> MLFAPTIKAQADTVPLPAPIIEAFPVEAIAEAIAGELDKDSVNDTITQADLDTMTAIPLPSLGLTGEDLSVLNNEVFTNAIELAIWSNNIGELPDLSEALPALENIEANGANITVFPDANYPNLTNVDLSQNNFGFNIPKFVGMEGLVSINMENAGLSGYIAEDIWMNMPNLDSLILNENHLISIPEDIFLSQQLGTHSFANQTATYPPTTIKQGENLKVFVPFIYQALDFIAPSNHDLIIIKDNGRTLYEPPYPTYDGSY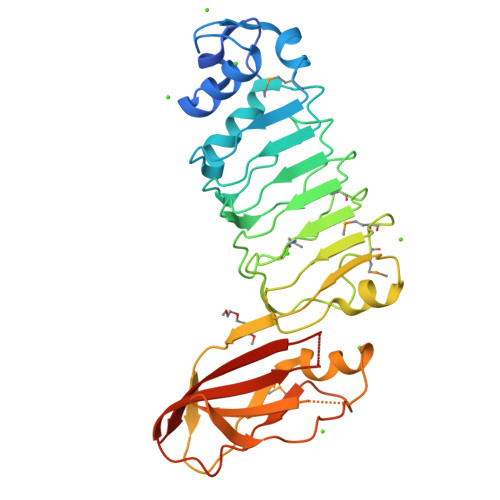MYTIETAGLQPGEHLLEISLGYNSGEYTGWYDFPVTITESNA>MTAPTVPVALVTGAAKRLGRSIAEGLHAEGYAVCLHYHRSAAEANALSATLNARRPNSAITVQADLSNVATAPVSGADGSAPVTL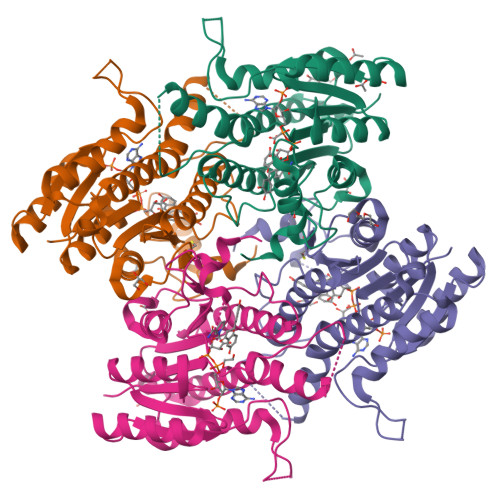FTRCAELVAACYTHWGRCDVLVNNASSFYPTPLLRNDEDGHEPCVGDREAMETATADLFGSNAIAPYFLIKAFAHRVAGTPAKHRGTNYSIINMVDAMTNQPLLGYTIYTMAKGALEGLTRSAALELAPLQIRVNGVGPGLSVLVDDMPPAVWEGHRSKVPLYQRDSSAAEVSDVVIFLCSSKAKYITGTCVKVDGGYSLTRA[4x]>[2x]MTSRKKVLLKVIILGDSGVGKTSLMNQYVNKKFSNQYKATIGADFLTKEVMVDDRLVTMQIWDTAGLERFQSLGVAFYRGADCCVLVFDVTAPNTFKTLDSWRDEFLIQASPRDPENFPFVVLGNKIDLENRQVATKRAQAWCYSKNNIPYFETSAKEAINVEQAFQTIARNALKQ;>GSMNTEAEQQLLHHARNGNAEE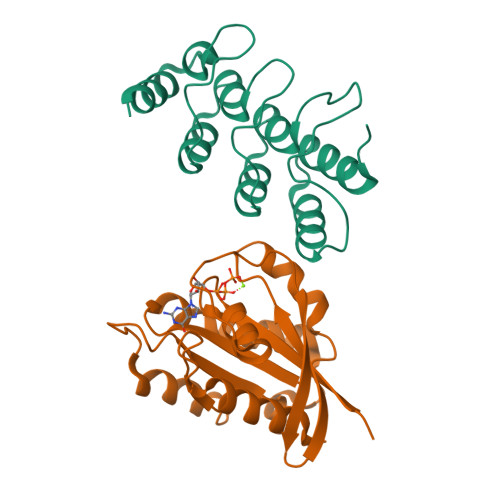VRKLLAAMARMEVVADIDCKGRSKSNLGWTPLHLACYFGHKQVVEDLLKAGAKVNMLNDMGDTPLHRAAFTGRKELVLLLLEYDADSTVVNGSGQTAKEATHDKEIRNMLEAVERT[2x]>[4x]AGVAKFAKYPLTFGPSPISNLNRLSQHLGSKVNVYAKREDCNSGLAFGGNKLRKL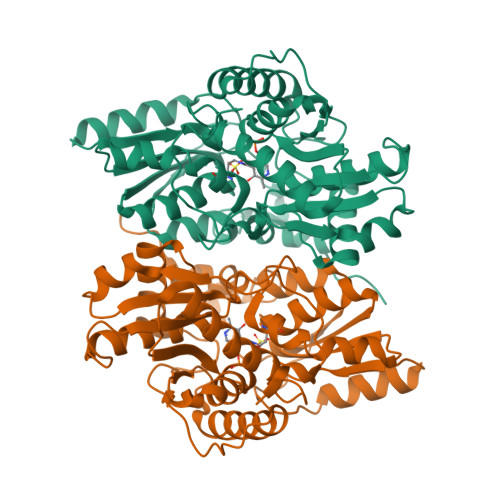EYIVPDIVEGDYTHLVSIGGRQSNQTRMVAALAAKLGKKCVLIQEDWVPIPEAEKDVYNRVGNIELSRIMGADVRVIEDGFDIGMRKSFANALQELEDAGHKPYPIPAGCSEHKYGGLGFVGFADEVINQEVELGIKFDKIVVCCVTGSTTAGILAGMAQYGRQDDVIAIDASFTSEKTKEQTLRIANNTAKLIGVEHEFKDFTLDTRFAYPCYGVPNEGTIEAIRTCAEQEGVLTDPVYEGKSMQGLIALIKEDYFKPGANVLYVHLGGAPALSAYSSFFPTKTA Tpp80Aa1 from Bacillus thuringiensis is a Toxin_10 family protein (Tpp) with reported action against Culex mosquitoes. We report the first crystal structure of Tpp80Aa1 at a resolution of 1.8 Å, which shows Tpp80Aa1 consists of two domains: an N-terminal β-trefoil domain resembling a ricin B lectin and a C-terminal putative pore-forming domain sharing structural similarity with the aerolysin family. We also identify that Tpp80Aa1 can interact with galactose-containing glycolipids and galactose, and this interaction is critical for exerting full insecticidal action against mosquito target cell lines. Here, we demonstrate an expanded target range, showing Tpp80Aa1 is also active against the larvae of Anopheles gambiae and Aedes aegypti mosquitoes.

Our final model had an Rwork/Rfree of 0.17/0.21 at 1.8 Å resolution and showed Tpp80Aa1 packs into the crystal lattice as homodimers, which could be indexed in the monoclinic space group C 1 2 1. The electron density map showed continuous density for residues 5–355 of the 373 aa wild-type Tpp80 protein sequence. Within each Tpp80Aa1 monomer, two distinct conserved domains appear: an N-terminal ricin B-lectin domain (IPR035992) spanning residues 5–155, and a C-terminal Toxin_10 domain (IPR008872) spanning residues 156–355. In the Tpp80Aa1 homodimer structure we also see the presence of two calcium ions (1 per monomer) and five buffer molecules present in the crystallization solution; four bis-tris propane and one citrate. The final model shows the presence of a homodimer with a large molecular interface forming an ‘X’ structure. In the case of Tpp80Aa1, PDBePISA interface analysis identified 12 interfaces; the largest interface (1010.9 Å2) between the two monomers in the ‘X’ shape involves 34 residues of monomer 1 and 35 residues of monomer 2, with 13 hydrogen bonds. Whereas the large Tpp1/Tpp2 interface may be preserved in solution, this is unlikely to be the case for the Tpp80Aa1 dimer—indeed SEC indicates Tpp80Aa1 is largely monomeric in solution. As Tpp80Aa1 does not need a partner to elicit toxicity, it is possible this ‘X’ shape is a requirement for packing and stability in the crystal structure. A structure reminiscent of an aerolysin insertion loop is present in Tpp80Aa1 between residues 259–272 (SWSIGADMGFS), as a short β-hairpin—with predominantly amphipathic structure—tucked under a loop. In Tpp80Aa1 we see a similar conservation (D73, Y88, S96, and E97) where the sidechains superimpose with those present in Tpp78Aa1, and we propose this as the putative galactose binding site of Tpp80Aa1.

>[2x]MGKSMTFKVGMKYMFKNKNSRKYLDISGNQTGNNANVQQYEYLADAPSERFFLHPLDNNYYAMINLNSGKVIDISGNQTSNNANIQQYEWLGDAPSEYWYFHREADGHYVIESKHSGKVLDIEGNQTGNNANVQQYEYLADAPSERFAVEEAGSVSLPSINTQPLSPVPQYETINDQLPEETERVVTAFTIVPAISVKDPHYGGDTAKQIKENPYYMVVKKQWWKKQESYVLAPSERYDFVTTTGIRVTDQETATKTVSWSIGADMGFSFKGFSMGMSSQYSQELQTSISHTTEQLKEETQEHHVTNPFLERMAYSRYILVTEYYVQRKNGTIVNAPWTMTDKTNAHAVTFPKSTGDLLNESTRKISKSESVK>[4x]HHHHHHMTDRVALRAGVPPFYVMDVWLAAAERQRTHGDLVNLSAGQPSAGAPEPVRAAAAAALHLNQLGYSVALGIPELRDAIAADYQRRHGITVEPDAVVITTGSSGGFLLAFLACFDAGDRVAMASPGYPC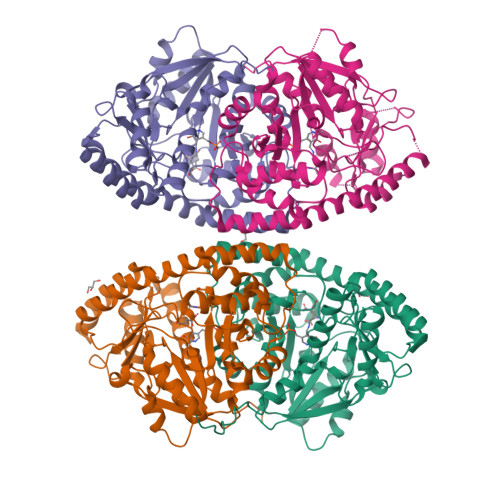YRNILSALGCEVVEIPCGPQTRFQPTAQMLAEIDPPLRGVVVASPANPTGTVIPPEELAAIASWCDASDVRLISDEVYHGLVYQGAPQTSCAWQTSRNAVVVNSFSKYYAMTGWRLGWLLVPTVLRRAVDCLTGNFTICPPVLSQIAAVSAFTPEATAEADGNLASYAINRSLLLDGLRRIGIDRLAPTDGAFYVYADVSDFTSDSLAFCSKLLADTGVAIAPGIDFDTARGGSFVRISFAGPSGDIEEALRRIGSWLPSQ(2-(4-(beta-L-fucopyranosylethynyl)phenyl)-2-methylpropan-1-amine 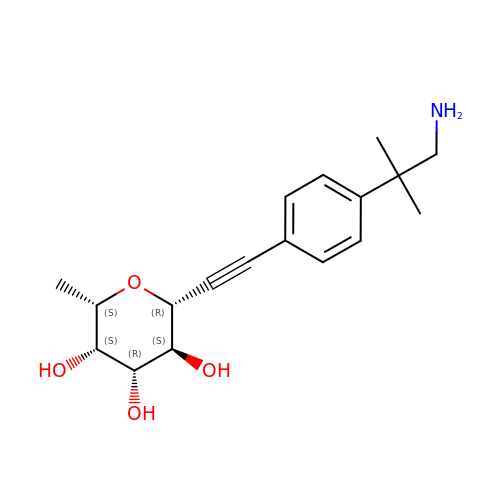| C18 H25 N O4 | OLKQUCDVBRXNDQ-WVRYCFJFSA-N>[4x]MAQDMSPRQSAEAFGVPAVSSSWVNQDGSTMTLVFGAGNSVSGFYVNNAPGFGCQGTPYPLVGLTWGNFIGFTVAW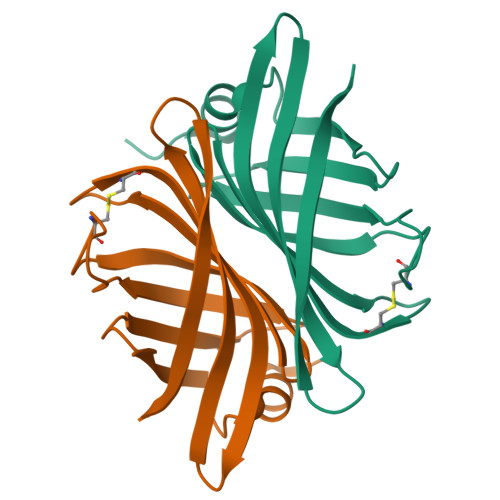DNATANCNSVTSWTGFAEAAGSDVTIVTDWNLAYQGSSSGEIQQGSDTFTLVNKAMK>MAAEDTPQDIADRERIFKRFDTNGDGKISSSEL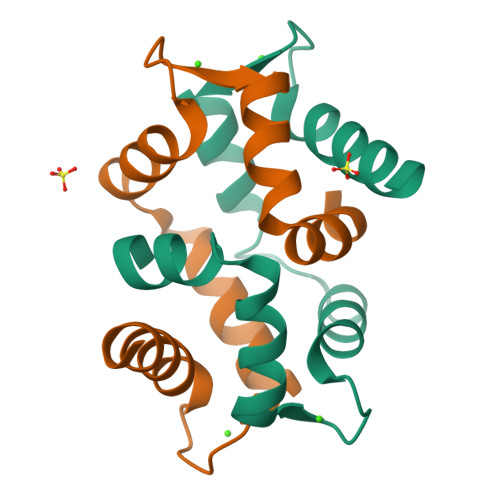GDALKTLGSVTPDEVRRMMAEIDTDGDGFISFDEFTDFARANRGLVKDVSKIF[4x]>[2x]GMKPHTLLIVDDDDTVAEMLELVLRGAGYEVRRAASGEEALQQIYKNLPDALICDVLLPGIDGYTLCKRVRQHPLTKTLPILMLTAQGDISA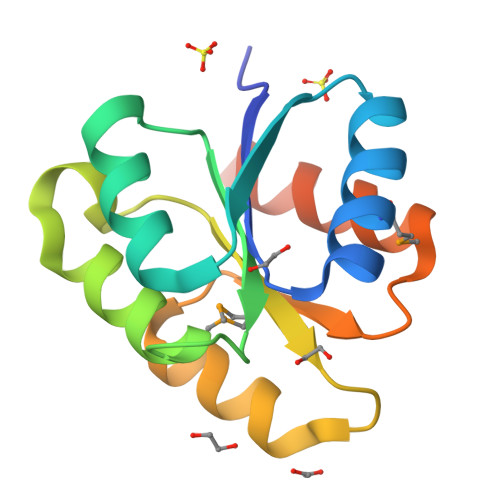KIAGFEAGANDYLAKPFEPQELVYRVKNILARTTIETPTTPVQR> MSILANKDTRAVIIGGVAGVNAAKRMAQFDFLVNRPLTVQAFVYPPEAGQQKEIFRGGELKNVTVYDSLAPALEEHPDINTALIYLGASRAAQAAKEALESPNIQLVSMITEGVPEKDAKRLKKLAQKLGKMLNGPSSIGIMSAGECRLGVIGGEFKNLKLCNLYRQGSFGVLTKSGGLSNEAMWLCAQNGDGITSAVAIGGDAYPGTDFVTYLEMFEKDPATKAVVMIGEVGGNLEEEAAEWLAAEPRRIKLIAAIGGTCQEVLPQGMKFGHAGAKEGKKGAGSARSKMNALRDAGAYVPDTFGGLSKEIKKVYEELIAAGEISTEIDEAVLPELPPRVQEVMKQGEVIVEPLIRT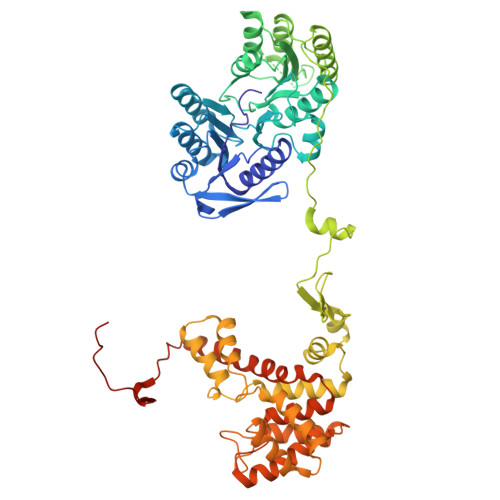TISDDRGEEPRYAGYAASELCSKGYGIEDVIGLLWNKKLPTREESEIIKRIVMISADHGPAVSGAFGSILAACAGIDMPQAVSAGMTMIGPRFGGAVTNAGKYFKMAVEDYPNDIPGFLSWMKKNVGPVPGIGHRVKSVKNPDQRVKYLVSYIKNETSLHTPCLDYALEVEKVTTAKKGNLILNVDGTIGCILMDLDFPVHSLNGFFVLARTIGMIGHWIDQNNQNSRLIRLYDYLINYAVKPEQEVPEKKGGSHHHHHH> LDEHCERLPYDASKWEFPRDRLKLGKPLGRGAFGQVI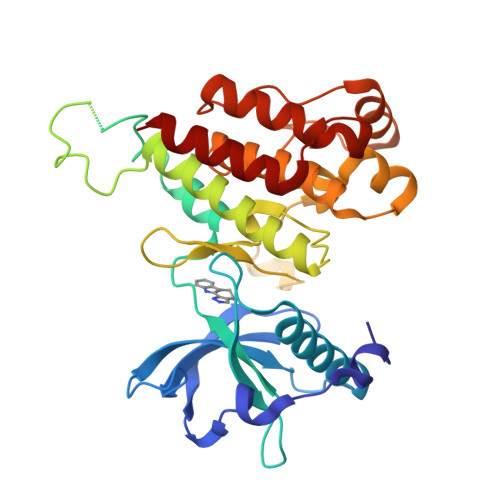EADAFGIDKTATCRTVAVKMLKEGATHSEHRALMSELKILIHIGHHLNVVNLLGACTKPGGPLMVIVEFCKFGNLSTYLRSKRNEFVPYKTKGARFRQGKDYVGAIPVDLKRRLDSITSSQSSASSGFVEEKSLSDVEEEEAPEDLYKDFLTLEHLICYSFQVAKGMEFLASRKCIHRDLAARNILLSEKNVVKICDFGLARDIYKDPDYVRKGDARLPLKWMAPETIFDRVYTIQSDVWSFGVLLWEIFSLGASPYPGVKIDEEFCRRLKEGTRMRAPDYTTPEMYQTMLDCWHGEPSQRPTFSELVEHLGNLLQANA> MRGSHHHHHHGSPGLQEFMAATGANAEKAESHNDCPVRLLNPNIAKMKEDILYHFNLTTSRHNFPALFGDVKFVCVGGSPSRMK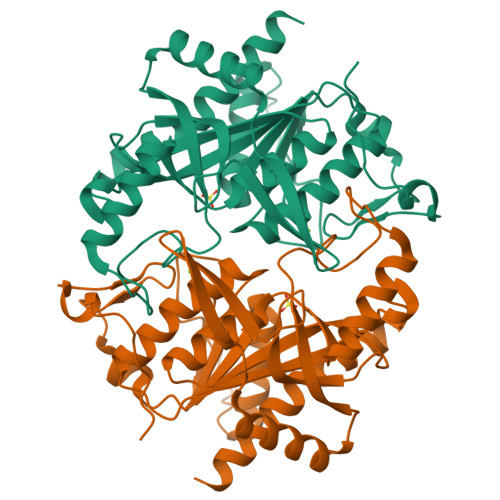AFIRCVGAELGLDCPGRDYPNICAGTDRYAMYKVGPVLSVSHGMGIPSISIMLHELIKLLYYARCSNVTIIRIGTSGGIGLEPGTVVITEQAVDTCFKAEFEQIVLGKRVIRKTDLNKKLVQELLLCSAELSEFTTVVGNTMCTLDFYEGQGRLDGALCSYTEKDKQAYLEAAYAAGVRNIEMESSVFAAMCSACGLQAAVVCVTLLNRLEGDQISSPRNVLSEYQQRPQRLVSYFIKKKLSKA(3S)-3-(2-amino-5-chloro-1H-benzimidazol-1-yl)-N-[(1R,3S,5R,7R)-tricyclo[3.3.1.1~3,7~]dec-2-yl]pentanamide | C22 H29 Cl N4 O | 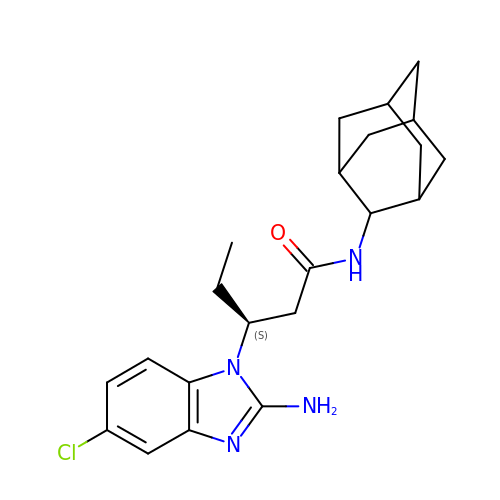KMAKOMVKNWTGPE-LIXZBVSLSA-N In this study, we identified that PH1991 is a tRNA:m5C72 MTase NSun6 (PhNSun6). In contrast to hNSun6, which could only methylate four tRNAs with U73, PhNSun6 could catalyze m5C72 formation on eleven PhtRNAs harboring either U73 or G73. PhNSun6, with 12 α-helices and 19 β-strands, is divided into two distinct domains with different sizes: the MTase domain, including an RRM motif (residues 34–79 and residues 173–185) and a Rossmann-fold catalytic core (residues 185–389), and the PUA domain (residues 86–164). The tRNA substrates recognized by PhNSun6 were based on (i) the 3′ CCA terminus, (ii) the target site C72, (iii) U73 or G73, and (iv) the discriminatory base pair C2:G71 at the acceptor stem.

To better understand the recognition mechanism of PhNSun6, we solved the crystal structures of PhNSun6 in the apo form and in complex with SAM, sinefungin (an analog of SAM, SFG), and S-adenosyl-homocysteine (demethylated SAM, SAH). Cofactors bind at the Rossmann-fold catalytic core of PhNSun6. When comparing the structures of PhNSun6 in the apo form and in the form bound with cofactors, the overall structures do not show distinct changes, except that helix α9 moves a slightly toward the cofactors. Residues Met208, Ala209, Pro279, Phe308, Asp260, Asp233, Arg238, Ala211, Asp277, Lys215, Tyr304, Gly213 and Gly214 form the binding pocket for the cofactor SAH, as shown in Figure 5B. In the PhNSun6-SAM and PhNSun6-SFG complexes, similar binding models of the cofactors to that of SAH were observed, but are not discussed here. Although PhNSun6 contains a different RNA recognition motif compared with that in hNSun6, the main structure of PhNSun6 adopts a similar topology to hNSun6 and the two active Cys residues of PhNSun6 are conserved. The two conserved Cys residues point from opposite site sides of the cofactor, which is the same as that in hNSun6.

>[2x]YLEAFPKELREYYKNLFGKEEANKIMKKLREPVEHYYIRVNTLKISREKLIGELKKEGLKPLRSPYLPEGLYFVREGPNFSDDFEPKLPVVVANKYAAESVYQGAMLYAPGVLKADKNIKEGDEVQIRDPKGLLVGIGIARMDYKEMTEATRGLAVEVTLPKFKLPSLSELKAFEKGYFYPQGLPSMVTARVLEPKEDDVIIDMAAAPGGKTTHIAQLLENKGEIIAIDKSKNRLRKMEENIKRLGVKNVKLVQMDARKLPDLGIKADKILLDAPCTALGVRPKLWEERTLKHIEATARYQRAFIWAAIKSLRRGGVLVYSTCTLSYEENEGNVKFMIRKGMKLEEQSIFIGSPGIGMNKVQRFYPHKHLTQGFFIAKLRKVKD[(2R)-2-{2-[hydroxy(methyl)amino]-2-oxoethyl}-5-(3-methylphenyl)pentyl]phosphonic 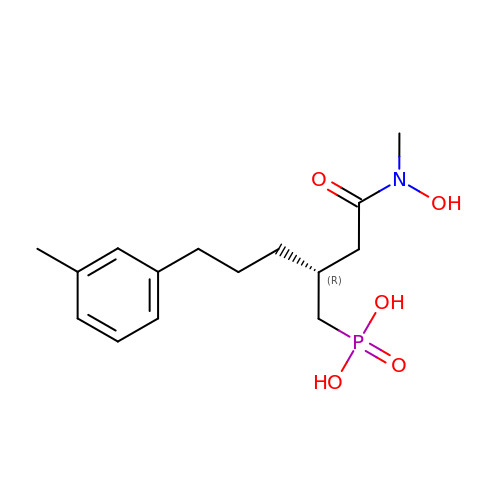acid | C15 H24 N O5 P | LKGTWQXFDFYGBW-CQSZACIVSA-N> ETPPRFTRTPVDQTGVSGGVASFICQATGDPRPKIVWNKKGKKVSNQRFEVIEFDDGSGSVLRIQPLRTPRDEAIYECVASNNVGEISVSTRLTVLREDQIPRGFPTIDMGPQLKVVERTRTATMLCAASGNPDPEITWFKDFLPVDTSNNNGRIKQLRSESIGGTPIRGALQIEQSEESDQGKYECVATNSAGTRYSAP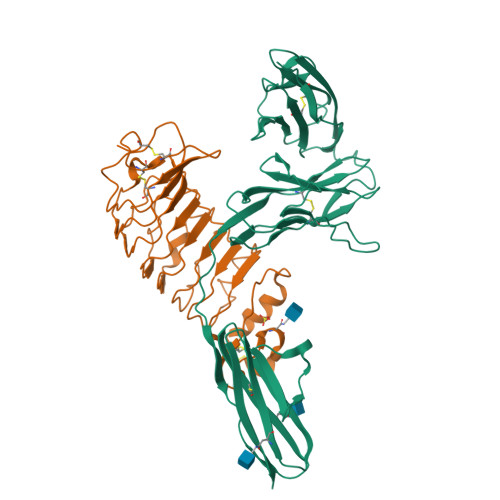ANLYVRELREVRRVPPRFSIPPTNHEIMPGGSVNITCVAVGSPMPYVKWMLGAEDLTPEDDMPIGRNVLELNDVRQSANYTCVAMSTLGVIEAIAQITVKALSRLVPR;> TGDVCKEKICSCNEIEGDLHVDCEKKGFTSLQRFTAPTSQFYHLFLHGNSLTRLFPNEFANFYNAVSLHMENNGLHEIVPGAFLGLQLVKRLHINNNKIKSFRKQTFLGLDDLEYLQADFNLLRDIDPGAFQDLNKLEVLILNDNLISTLPANVFQYVPITHLDLRGNRLKTLPYEEVLEQIPGIAEILLEDNPWDCTCDLLSLKEWLENIPKNALIGRVVCEAPTRLQGKDLNETTEQDLCPLKSRLVPR>[2x]GPLGSYSHTATPAITLPSSGSANFAGVEYPLLPLDQHTPLLFQWFERNPSRFGENQIPIINTQQNPYLNNIINAAIIEKERTIGVLVDGNFSAGQKKALAKLEKQYENIKVIYNSDLDYSMYDKKLSDIYLENIAKIEAQPANVRDEYLLGEIKKSLNEVLKNNPEESLVSSHDKRLGHVRFDFYRNLFLLKGSNAFLEAGKHGCHHLQPGGGCIYLDADMLLTGKLGTLYLPDGIAVHVSRKGNSMSLENGIIAVNRSEHPALKKGLEIMHSKPYGDPYIDGVCGGLRHYFNCSIRHNYEEFCNFIEFKHEHIFMDTSSLTISSWR

Three highly related Salmonella effectors, SseK1, SseK2, and SseK3, orthologues of the enteropathogenic and enterohemorrhagic Escherichia coli T3SS effector NleB1 (7), translocate via the T3SS into the host cell. Similarly to NleB1 (9, 10), SseK1 and SseK3 are N-acetylglucosamine (GlcNAc) transferases that modify the TNFR1-associated death domain protein TRADD and inhibit activation of the pro-inflammatory transcription factor NF-κB, as well as necroptotic host cell death. Here we report the structure of the Salmonella arginine N-glycosyltransferase, SseK3, in its apo and ligand-bound forms. The SseK3 catalytic core domain (∼250 residues) shows the classic features of the large glycosyltransferase type-A family of enzymes (GT-A) consisting of a single module composed of a central parallel β-sheet core flanked by a number of α-helices.

The structure of SseK3(14–335) at 2.20 Å in complex with UDP, GlcNAc, and Mn2+ was solved by molecular replacement using the apo-structure. Due to the length of the crystallization process and to the hydrolysis capabilities of SseK3(14–335), in the structure co-crystallized in the presence of UDP-GlcNAc and Mn2+, the ligand is hydrolyzed with the UDP and N-acetyl α-d-glucosamine still present in the active site. A comparison with the apo-structure reveals that the C-terminal amino acids in the ligand-bound SseK3 fold back onto the ligand to produce a short segment of α-helix, with the last two residues Trp-334 and Arg-335 directly interacting with the UDP and GlcNAc. SseK3 contains the classic GT-A DXD motif (226DAD228) that coordinates the divalent manganese cation in an octahedral geometry. Mn2+ interacts with the carboxylate oxygens of Asp-228 and Asp-325, the UDP diphosphate, and the hydroxyl group of Ser-327, as well as an ordered water molecule, which bridges, via hydrogen bonds, the metal atom and the carboxyl group of Asp-226 of the DXD motif. Ser-333, Trp-334, and Arg-335 all interact via hydrogen bonds with the oxygen atoms of the diphosphate. The last residue visible in the structure of SseK3(14–333), serine 332, translates 17 Å from its position in the apo-structure to interact directly with a β-oxygen of the UDP. The N-acetyl α-d-glucosamine in the active site is stabilized by a series of interactions that involve the anomeric C1 hydroxyl group, at a distance of 3.6 Å from the phosphorus atom to which it was bound, and the guanidine group of Arg-335, with hydrophobic interactions also established between the sugar and the aromatic ring of Trp-334. The GlcNAc C4 and C6 hydroxyl groups in the structure of ligand-bound SseK3 are locked in the active site by the side-chain carboxylate of Asp-191, which may explain why UDP-Gal, which has a C4 inverted stereochemistry compared with glucose, shows the lowest affinity for SseK3. Differently from the clostridial toxins, the active site in SseK3 contains a glutamic acid residue, Glu-258, 3.2 Å away from the anomeric carbon.>[2x]MKISVSKNDLENALRYLQAFLDKKDASSIASHIHLEVIKEKLFLKASDSDIGLKSYIFTQSSDKEGVGT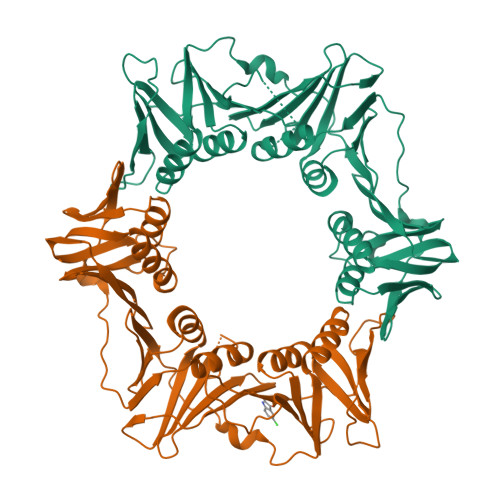INGKKFLDIISCLKDSNIILETKDDSLAIKQNKSSFKLPMFDADEFPEFPVIDPKVSIEVNAPFLVDAFKKIAPVIEQTSHKRELAGILMQFDQKHQTLSVVGTDTKRLSYTQLEKISIHSTEEDISCILPKRALLEILKLFYENFSFKSDGMLAVIENEMHTFFTKLIDGNYPDYQKILPKEYISSFTLGKEEFKESIKLCSSLSSTIKLTLEKNNALFESLDSEHSETAKTSVEIEKGLDIEKAFHLGVNAKFFLEALNALGTTQFVLRCNEPSSPFLIQESLDEKQSHLNAKISTLMMPITL>MTAQPNSLEARDIRYHLHSYTDAVRLEAEGPLVIERGDGIYVEDVSGKRYIEAMSGLLSVGVGFSEPRLAEAAARQMKKLPFYHTFSYRSHGPVIDLAEKLVSMAPVPMSKAYFTNSGSEANDTVVKLIWYRSNALGEPERKKIISRKRGYHGVTIASASLTGLPNNHRSFDLPIDRILHTGCPHFYREGQAGESEEQFATRLADELEQLIIAEGPHTIAAFIGEPVM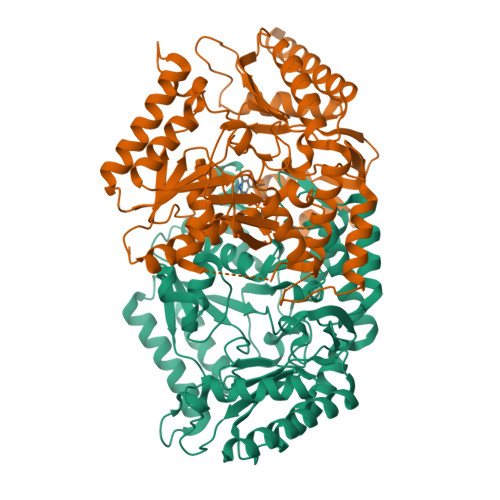GAGGVVVPPKTYWEKVQAVLKRYDILLIADEVICGFGRTGNLFGSQTFDMKPDILVMSKQLSSSYLPISAFLINERVYAPIAEESHKIGTLGTGFTASGHPVAAAVALENLAIIEERDLVANARDRGTYMQKRLRELQDHPLVGEVRGVGLIAGVELVTDKQAKTGLEPTGALGAKANAVLQERGVISRAMGDTLAFCPPLIINDQQVDTMVSALEATLNDVQASLTR[2x]> NDYCQHFVDTGHRPQNFIRDVGLADRFEEYPKLRELIRLKDELIAKSNTPPMYLQADIEAFDIRELTPKFDVILLEPPLEEYYRETGITANEKCWTWDDIMKLEIDEIAAPRSFIFLWCGSGEGLDLGRVCLRKWGYRRCEDICWIKTNKNNPGKTKTLDPKAVFQR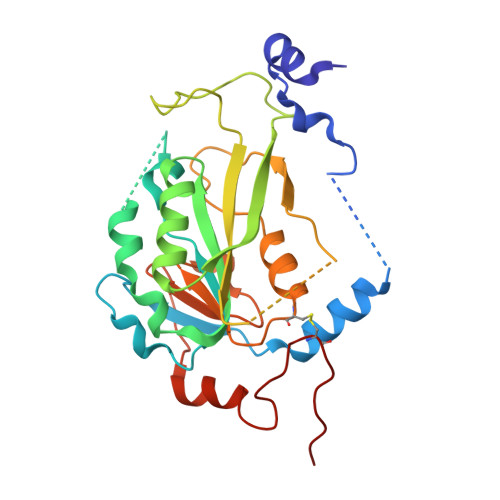TKEHCLMGIKGTVKRSTDGDFIHANVDIDLIITEEPEIGNIEKPVEIFHIIEHFCLGRRRLHLFGRDSTIRPGWLTVGPTLTNSNYNAETYASYFSAPNSYLTGCTEEIERL>[2x]GGLEKDFLPLYFGWFLTKKSSETLRKAGQVFLEELGNHKAFKKELRHFISGDEPKE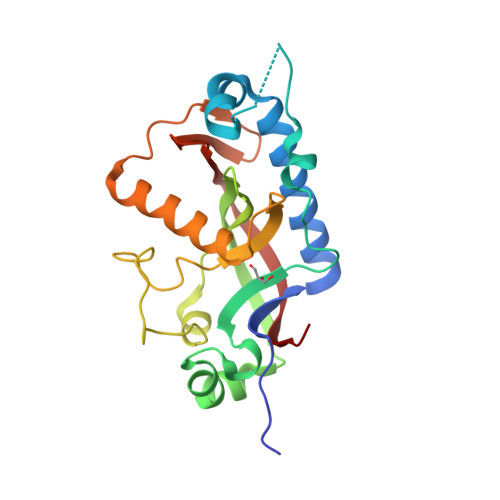KLELVSYFGKRPPGVLHCTTKFCDYGKAAGAEEYAQQEVVKRSYGKAFKLSISALFVTPKTAGAQVVLTDQELQLWPSDLDKPSASEGLPPGSRAHVALGCAADVQPVQTGLDLLDILQQVKGGSQGEAVGELPRGKLYSLGKGRWMLSLTKKMEVKAIFTGYYG>MIFMFRKVLFPTDFSEGAYRAVEVFEKRNKMEVGEVILLHVIDEGTLEELMDGYSFFYDNAEIELKDIKEKLKEEASRKLQEKAEEVKRAFRAKNVRTIIRFGIPWDEIVKVAEEENVSLIILPSRGKLSLSHEFLGSTVMRVLRKTKKPVLIIKEVDENELAKTKGTSG[4x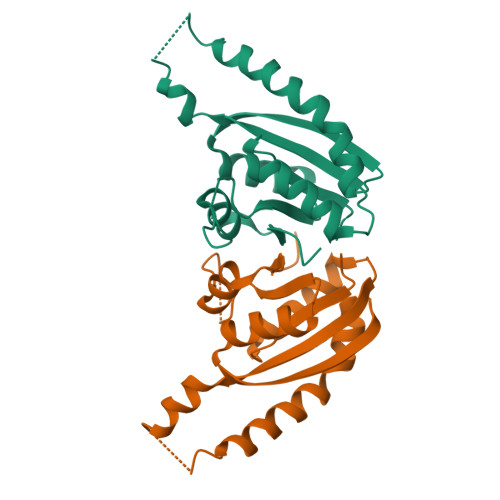]>MAQILPIRFQEHLQLQNLGINPANIGFSTLTMESDKFICIREKVGEQAQVVIIDMNDPSNPIRRPISADSAIMNPASKVIALKAGKTLQIFNIEMKSKMKAHTMTDDVTFWKWISLNTVALVTDNAVYHWSMEGESQPVKMFDRHSSLAGCQIINYRTDAKQKWLLLTGISAQQNRVVGAMQLYSVDRKVSQPIEGHAASFAQFKMEGNAEESTLFCFAVRGQAGGKLHIIEVGTPPTGNQPFPKKAVDVFFPPEAQNDFPVAMQISEKHDVVFLITKYGYIHLYDLETGTCIYMNRISGETIFVTAPHEATAGIIGVNRKGQV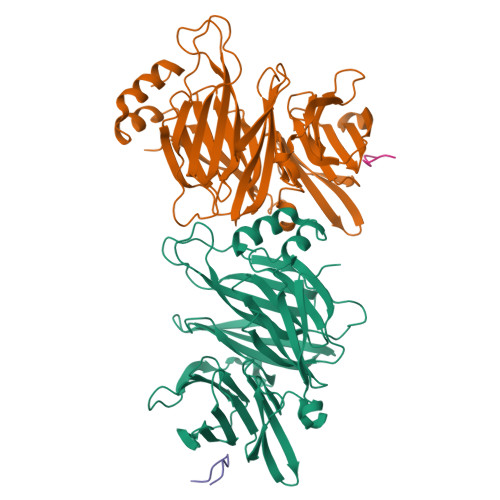LSVCVEEENIIPYITNVLQNPDLALRMAVRNNLAG[2x];>[2x]AVSLLDLDA>GLSSSPSEILQELGKGSTHPQPGVSPPAAPAAPGPKDGPGETDAFGNSEGKELVASGENKIKQGLLPSLEDLLFYTIAEGQEKIPVHKFITALKSTGLRTSDPRLKECMDMLRLTLQTTSDGVMLDKDLFKKCVQSNIVLLTQAFRRKFVIPDFMSFTSHIDELYESAKKQSGGKVADYIPQLAKFSPDLWGVSVCTVDGQRHSTGDTKVPFCLQSCVKPLKYAIAVNDLGTEYVHRYVGKEPSGLRFNKLFLNEDDKPHNPMVNAGAIVVTSLIKQGVNNAEKFDYVMQFLNKMAGNEYVGFSNATFQSERESGDRNFAIGYYLKEKKCFPEGTDMVGILDFYFQLCSIEVTCESASVMAATLANGGFCPITGERVLSPEAVRNTLSLMHSCGMYDFSGQFAFHVGLPAKSGVAGGILLVVPNVMGMMCWSPPLDKMGNSVKGIHFCHDLVSLCNFHNYDNLRHFAK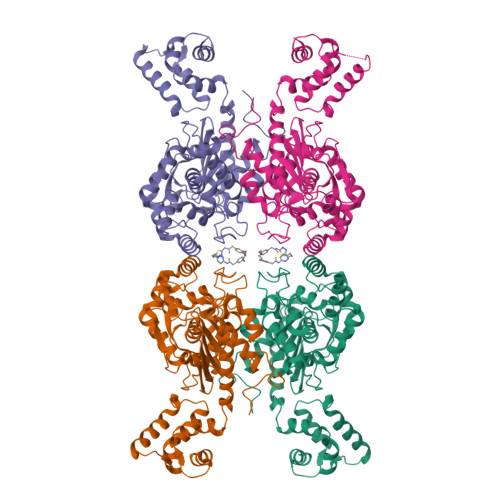KLDPRREGGDQRHSFGPLDYESLQQELALKETVWKKVSPESNEDISTTVVYRMESLGEKSHHHHHH[4x]>MWIIEAEGDILKGKSRILFPGTYIVGRNVSDDSSHIQVISKSISKRHARFTILTPSEKDYFTGGPCEFEVKDLDTKFGTKVNEKVVGQNGDSYKEKDLKIQLGKCPFTINAYWRSMCIQFDNPEMLSQWASNLNLLGIPTGLRDSDATTHFVMNRQAGSSITVGTMYAFLKKTVIIDDSYLQYLSTVKESVIEDASLMPDALECFKNIIKNNDQFPSSPEDCINSLEGFSCAMLNTSSESHHLLELLGLRISTFMSLGDIDKELISKTDFVV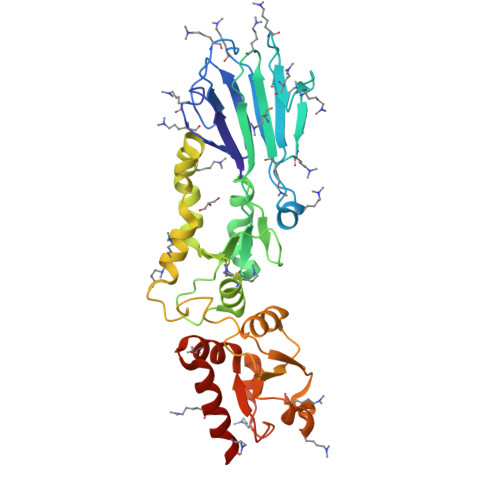LNNAVYDSEKISFPEGIFCLTIEQLWKIIIERNSRELISKEIERLKYATASN[2x]>[3x]MAAQIPESDQIKQFKEFLGTYNKLTETCFLDCVKDFTTREVKPEETTCSEHCLQKYLKMTQRISMRFQEYHIQQNEALAAKAGLLGQPR;>[3x]MDPLRAQQLAAELEVEMMADMYNRMTS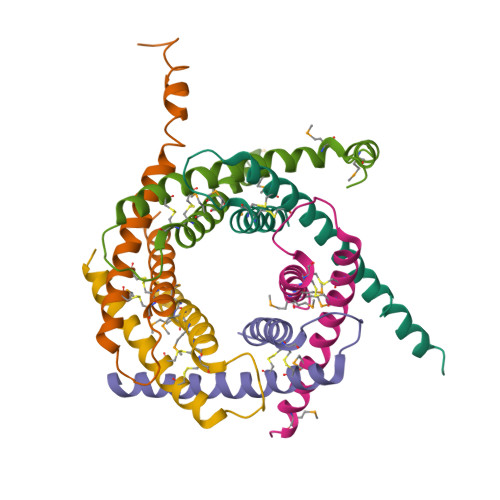ACHRKCVPPHYKEAELSKGESVCLDRCVSKYLDIHERMGKKLTELSMQDEELMKRVQQSSGPA>VSEDLRSRIEVLKRKVIEKVQHIQLLQKNVRAQLVDMKRLEVDIDIKIRSCRGSCSRALAREVDLKDYEDQQKQLEQVIAKDLLPSR[2x];>[2x]DNENVVNEYSSELEKHQLYIDETVNSNIPTNLRVLRSILENLRSKIQKLESDVSAQMEYCRTPCTVSCNIPVVSGKECEEIIRKGGETSEMYLIQPDSSVKPYRVYCDMNTENGGWTVIQNRQDGSVDFGRKWDPYKQGFGNVATNTDGKNYCGLPGEYWLGNDKISQLTRMGPTELLIEMEDWKGDKVKAHYGGFTVQNEANKYQISVNKYRGTAGNALMDGASQLMGE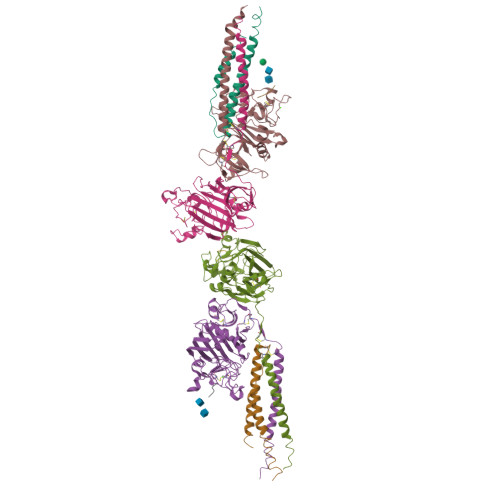NRTMTIHNGMFFSTYDRDNDGWLTSDPRKQCSKEDGGGWWYNRCHAANPNGRYYWGGQYTWDMAKHGTDDGVVWMNWKGSWYSMRKMSMKIRPFFPQQ;>KMLEEIMKYEASILTHDSSIRYLQEIYNSNNQKIVNLKEKVAQLEAQCQEPCKDTVQIHDITGKDCQDIANKGAKQSGLYFIKPLKANQQFLVYCEIDGSGNGWTVFQKRLDGSVDFKKNWIQYKEGFGHLSPTGTTEFWLGNEKIHLISTQSAIPYALRVELEDWNGRTSTADYAMFKVGPEADKYRLTYAYFAGGDAGDAFDGFDFGDDPSDKFFTSHNGMQFSTWDNDNDKFEGNCAEQDGSGWWMNKCHAGHLNGVYYQGGTYSKASTPNGYDNGIIWATWKTRWYSMKKTTMKIIPFNRLTIGEGQQHHLGGAKQAGDV[2x];>[2x]GPR;>[2x]GHRPLDK> MRSYLILRLAGPMQAWGQPTFEGTRPTGRFPTRSGLLGLLGACLGIQRDDTSSLQALSESVQFAVRCDELILDDRRVSVTGLRDYHTVLGAREDYRGLKSHETIQTWREYLCDASFTVALWLTPHATMVISELEKAVLKPRYTPYLGRRSCPLTHPLFLGTCQASDPQKALLNYEPVGGDIYSEES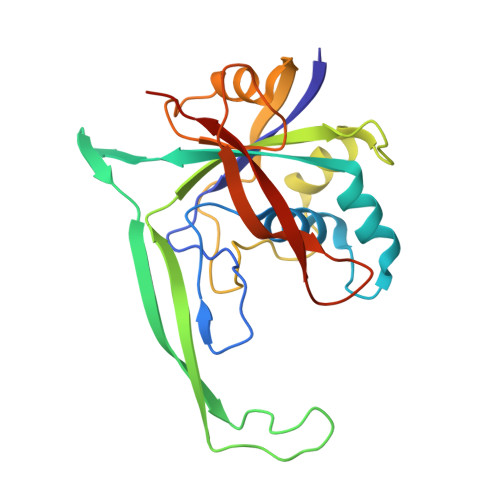VTGHHLKFTARDEPMITLPRQFASREWYVIKGGMDVSQ>MSFDLIIKNGTVILENEARVVDIAVKGGKIAAIGQDLGDAKEVMDASGLVVSPGMVDAHTHISEPGRSHWEGYETGTRAAAKGGITTMIEMPLNQLPATVDRASIELKFDAAKGKLTIDAAQLGGLVSYNIDRLHELDEVGVVGFKCFVATCGDRGIDNDFRDVNDWQFFKGAQKLGELGQPVLVHCENALICDELGEEAKREGRVTAHDYVASRPVFTEVEAIRRVLYLAKVAGCRLHVCHVSSPEGVEEVTRARQEGQDVTCESCPHYFVLDTDQFEEIGTLAKCSPPIRDLENQKGMWEKLFNGEIDCLVSDHSPCPPEMKAGNIMEAWGGIAGLQNCMDVMFDEAVQKRGMSLPMFGKLMATNAADIFGLQQKGRIAPGKDADFVFIQPNSSYVLTNDDLEYRHKVSPYVGRTIGARITKTILRGDVIYDIEQGFPVAPKGQFILKHQQHHHHHH[4x]

Allantoinase (ALLase; EC 3.5.2.5) possesses a binuclear metal center in which two metal ions are bridged by a posttranslationally carbamylated lysine. ALLase catalyzes the reversible conversion of allantoin to allantoic acid by hydrolytic cleavage of the five-member hydantoin ring. This ALLase-catalyzed reaction is a key process in the biosynthesis and degradation of ureide required for the utilization of nitrogen in purine-derived compounds. ALLase is a member of the cyclic amidohydrolase family, which also includes dihydroorotase (DHOase), dihydropyrimidinase (DHPase), hydantoinase (HYDase), and imidase.

We crystallized EcALLase-BL21 and determined its structure at a resolution of 2.07 Å. Four monomers of EcALLase-BL21 per asymmetric unit were present. The global architecture of EcALLase-BL21 revealed a TIM-barrel structure that consisted of 17 α-helices, 20 β-sheets, and 2 Zn ions. The active site of EcALLase-BL21 containing H59, H61, Kcx146, H186, H242, and D315, which were required for the metal binding, was similar to that of EcALLase-K12 and other members of the cyclic amidohydrolase family, such as Pseudomonas aeruginosa DHPase (PaDHPase) and the dihydroorotase domain of human CAD protein (huDHOase). The EcALLase-K12 structure had been solved, but three segments, including the two active site loops, namely aa 64–68 and 150–161, in the ternary structure, were undetermined. In this study, these two active site loops of EcALLase-BL21 were fully solved structurally. Based on our structure, the bottleneck size of the active site pocket of EcALLase-BL21 was approximately 3 Å. Given that the tunnel bottleneck (~3 Å) is narrower than the size of substrate allantoin (6–9 Å), this structure may be the closed form of EcALLase-BL21. Correspondingly, these residues in EcALLase-BL21 are E64 (loop I), G66 (loop I), F148 (loop II), T151 (loop II), and F161 (loop II). Accordingly, these amino acid residues on the dynamic loops may be also critical and can be modulated by rational design for the substrate specificity of EcALLase-BL21.Human mitochondrial nuclease EXOG (hEXOG) is important for mtDNA integrity. hEXOG depletion selectively increases lesions in mtDNA, but has no effect on chromosomal DNA. Human EXOG shares sequence homology with members of ββα-Me nuclease family, which contains nonspecific endonucleases. The catalytic Core domain of hEXOG is identical to EndoG, but its C-terminal extension forms a unique Wing domain that converts the enzyme from a nonspecific endonuclease into a DNA-geometry-specific exonuclease. Conversely, in mitochondrial LP-BER, the nuclease reaction occurs before DNA synthesis: hEXOG processes the 5′-end of DNA downstream of the lesion, generating an optimal substrate for DNA synthesis catalysed by Pol γ.

Apo hEXOG is a symmetrical homodimer. Each monomer contains a Core domain that is extremely similar to that of EndoG (r.m.s.d.=0.8 Å), and a helical-bundle Wing domain that corresponds to the C-terminal extension. The N terminus of each hEXOG monomer undergoes a domain-swap where the folding of the region is identical to that in EndoG, but the involved residues are from the opposing monomer rather than from the same monomer in EndoG: the residues 58KAVLEQFGFPLT70 (hydrophobic residues are bold) of one monomer collapse on a hydrophobic patch (277GLVFFPHL284) of the opposing monomer 30 Å away. A Mg2+ is found in each active site, forming octahedron coordination with five water molecules and Nδ of N171. The nature of Mg2+ was confirmed by Mn2+ substitution and single-wavelength anomalous dispersion data. In contrast to the completely solvent exposed active site of EndoG, the active site of hEXOG is an enclosed V-shaped cleft. The cleft, measuring 32–35 Å in depth and 15 Å in width, is lined with positively charged residues from both Core and Wing domains, and is both electrostatically and dimensionally capable of accommodating dsDNA at its end.

>MKAVLEQFGFPLTGTEARCYTNHALSYDQAKRVPRWVLEHISKSKIMGDADRKHCKFKPDPNIPPTFSAFNEDYVGSGWSRGHMAPAGNNKFSSKAMAETFYLSNIVPQDFDNNSGYWNRIEMYCRELTERFEDVWVVSGPLTLPQTRGDGKKIVSYQVIGEDNVAVPSHLYKVILARRSSVSTEPLALGAFVVPNEAIGFQPQLTEFQVSLQDLEKLSGLVFFPHLDRTSDIRNICSVDTCKLLDFQEFTLYLSTRKIEGARSVLRLEKIMENLKNAEIEPDDYFMSRYEKKLEELKAKEQSGTQIRKPSHHHHHH[2x]>[6x]MFENVSTFEEAFNKLLKEVLEFNLENPFEDAKKVICIEPHPDDCAIGMGGTIKKLSDEGVEVIYICMTDGYMGTTDEKLSGHELALIRRREEEESAKLLGVRKIYWLNYRDTELPYSREVRKDLVKII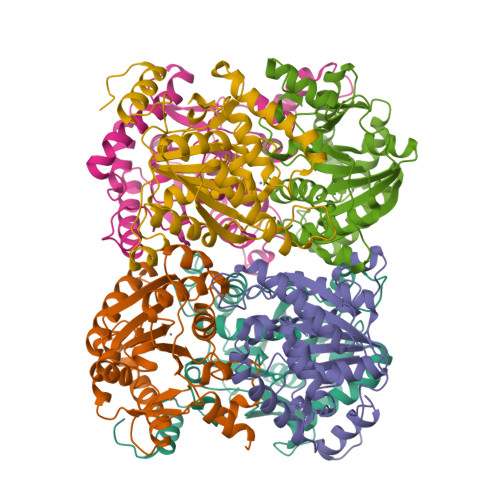RKEKPDGVFAPDPWLPYESHPDHRRTGFLAIESVAFSQLPNFSNIDIDIGLKPHSVSFIALYYTHKPNYIVDITDLMELKLKAIRAHRSQFTDDIWETWEPFLRTVTMFYGEKIGVRYGEGFRVMPGLFYHITPFADLI>[2x]MDNS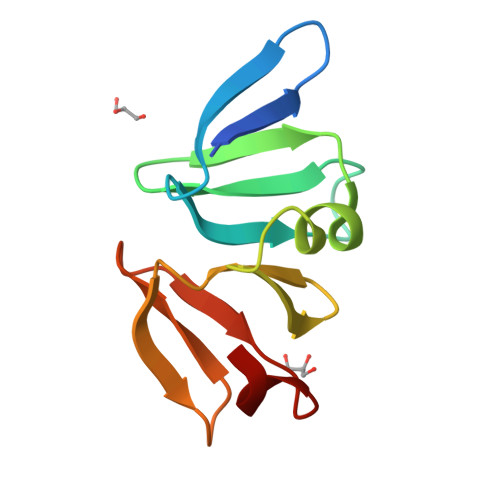VETIELKRGSNSVYVQYDDIMFFESSTKSHRLIAHLDNRQIEFYGNLKELSQLDDRFFRCHNSFVVNRHNIESIDSKERIVYFKNKEHCYASVRNVKKI>MVVKFMDVYQRSYCHPI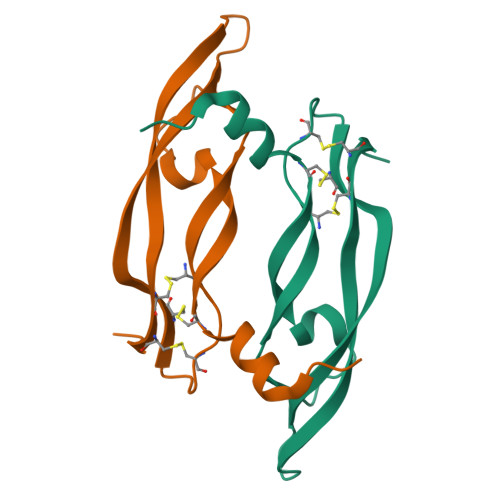ETLVDIFQEYPDEIEYIFKPSAVPLMRCGGACNDEGLECVPTEESNITMQIMRIKPHQGQHIGEMSFLQHNKCECRPKK[2x]> SGIVQQQNNLLRAIEAQQHLLQLTVWGIKQLQARILSGGSGGWMEWDREINNYTSLIHSLIEESQNQQEKNEQELLGGSGGSGIVQQQNNLLRAIEAQQHLLQLTVWGIKQLQARILSGGSGGWMEWDREINNYTSLIHSLIEESQNQQEKNEQELLGGSGGSGIVQQQNNLLRAIEAQQHLLQLTVWGIKQL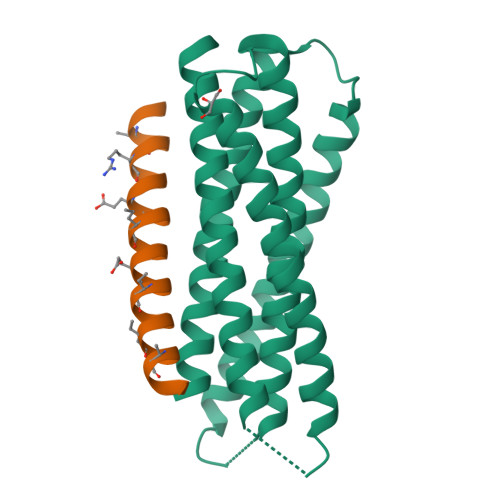QARIL;> XRTWEEWDRAIAEYARRIEELIRAAQEQQRKNEEALREL> MNNQPQGTNSVPNSIGNIFSNIGTPSFNMAQIPQQLYQSLTPQQLQMIQQRHQQLLRSRLQQQQQQQQQTSPPPQTHQSPPPPPQQSQPIANQSATSTPPPPPAPHNLHPQIGQVPLAPAPINLPPQIAQLPLATQQQVLNKLRQQAIAKNNPQVVNAITVAQQQVQRQIEQQKGQQTAQTQLEQQRQLLVQQQQQQQLRNQIQRQQQQQFRHHVQIQQQQQKQQQQQQQHQQQQQQQQQQQQQQQQQQQQQQQQQQQQQQQQQQQQQGQIPQSQQVPQVRSMSGQPPTNVQPTIGQLPQLPKLNLPKYQTIQYDPPETKLPYPTYWSDKKADTDTLLYEQIIQRDKINKYSLIRETNGYDPFSIYGFSNKEYISRLWHTLKYYQDLKNTRMKSITSTSQKIPSASIWGNGYSGYGNGITNTTTRVIPQVEVGNRKHYLEDKLKVYKQAMNETSEQLVPIRLEFDQDRDRFFLRDTLLWNKNDKLIKIEDFVDDMLRDYRFEDATREQHIDTICQSIQEQIQEFQGNPYIELNQDRLGGDDLRIRIKLDIVVGQNQLIDQFEWDISNSDNCPEEFAESMCQELELPGEFVTAIAHSIREQVHMYHKSLA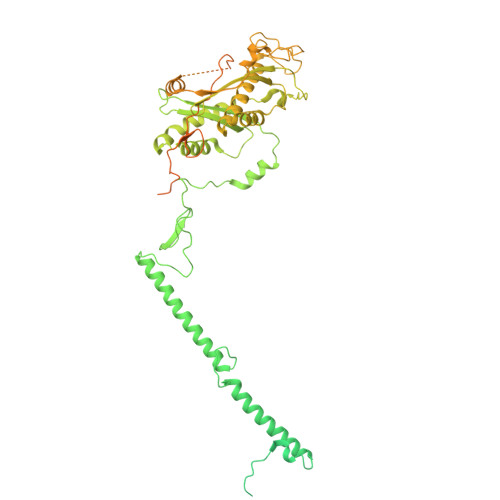LLGYNFDGSAIEDDDIRSRMLPTITLDDVYRPAAESKIFTPNLLQISAAELERLDKDKDRDTRRKRRQGRSNRRGMLALSGTSASNTSMNGVHNTVAAGNASSLPPGEILLPDIADIPRTFRTPVPSTLMPGGVDVGPSVESYELRNTTTYKSRPDRPKPVSPPCYIIDHIPGHSLLLSIKLPGKVNTKEEFAAAPNDTSSGTNAMLPSPESLKTKLNSNIRAGVTIPSIPNPIANHTVTNSPNPTLQPVIPGGAASKSVPTPSLPIAPPVAPHDSEATLLTNSNNGSSNNNTQNT> EVDEYMKEAVDHYAGQLMSLDINTEQMCLEDAMYGTDGLEALDLSTSAGYPYVAMGKKKRDILNKQTRDTKEMQKLLDTYGINLPLVTYVKDELRSKTKVEQGKSRLIEASSLNDSVAMRMAFGNLYAAFHKNPGVITGSAVGCDPDLFWSKIPVLMEEKLFAFDYTGYDASLSPAWFEALKMVLEKIGFGDRVDYIDYLNHSHHLYKNKTYCVKGGMPSGCSGTSIFNSMINNLIIRTLLLKTYKGIDLDHLKMIAYGDDVIASYPHEVDA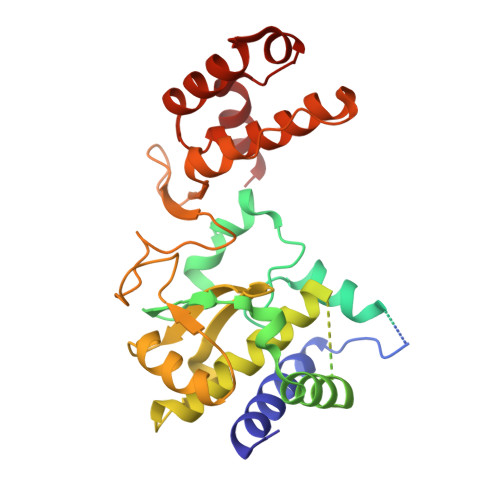SLLAQSGKDYGLTMTPADKSATFETVTWENVTFLKRFFRADEKYPFLIHPVMPMKEIHESIRWTKDPRNTQDHVRSLCLLAWHNGEEEYNKFLAKIRSVPIGRALALPEYSTLYDRWLDSF(2R,3R)-4-amino-N-[(1R,2S,3R,4R,5S)-5-amino-4-[(2,6-diamino-2,3,4,6-tetradeoxy-alpha-D-erythro-hexopyranosyl)oxy]-3-{[3-O-(2,6-diamino-2,3,4,6-tetradeoxy-beta-L-threo-hexopyranosyl)-beta-D-ribofuranosyl]oxy}-2-hydroxycyclohexyl]-3-fluoro-2-hydroxybutanamide 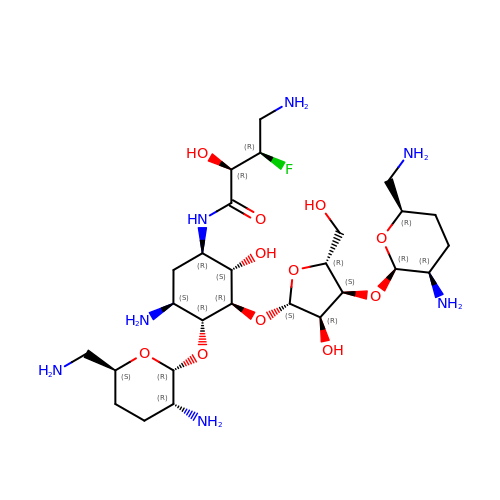| C27 H52 F N7 O11 | XWTWBGQMVSXRIE-ZLDKHCKJSA-N>[4x]TYGGYLRLDQLLSAQQPLSEPAHHDEMLFIIQHQTSELWLKLLAHELRAAIVHLQRDEVWQCRKVLARSKQVLRQLTEQWSVLETLTPSEYMGFRDVLGPSSGFQSLQYRYIEFLLGNKNPQMLQVFAYDPAGQARLREVLEAPSLYEEFLRYLARFGHAIPQQYQARDWTAAHVADDTLRPVFERIYENTDRYWREYSLCE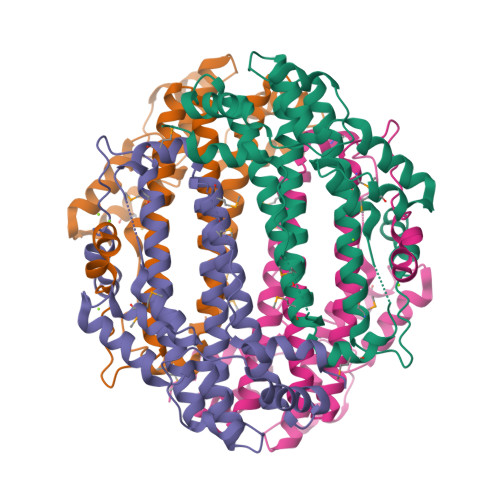DLVDVETQFQLWRFRHMRTVMRVIGFKRGTGGSSGVGFLQQALALTFFPELFDVRTSVGVDNRPPQGSADAGKR>[4x]MG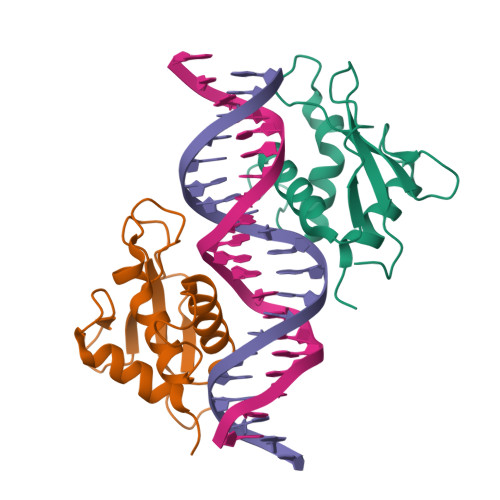SHHHHHHSAALEVLFQGPGGNGKLRQWLIDQIDSGKYPGLVWENEEKSIFRIPWKHAGKQDYNREEDAALFKAWALFKGKFREGIDKPDPPTWKTRLRCALNKSNDFEELVERSQLDISDPYKVYRIVPEGAKKGAKQL2-azanyl-9-[(2~{R},3~{R},4~{S})-3-oxidanyl-4-[oxidanyl-bis(oxidanylidene)-$l^{6}-phosphanyl]oxy-oxolan-2-yl]-1~{H}-purin-6-one 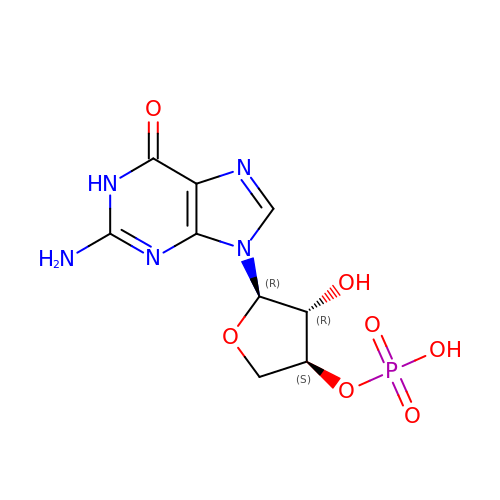| C9 H11 N5 O7 P | RGZPMPBDCRFFGY-OTEWCHCRSA-N>MATETTKMIYTPPPLDIKMEIEIGEQPQPPVKCSNFFANHWKGLVVFLVPLLCLPVMLLNEGAEFRCMYLLLVMAIFWVTEALPLYVTSMIPIVAFPIMGIMSSDQTCRLYFKDTLVMFMGGIMVALAVEYCNLHKRLALRVIQIVGCSPRRLHFGLIMVTMFLSMWISNAACTAMMCPIIQAVLEELQAQGVCKINHEPQYQIVGGNKKNNEDEPPYPTKITLCYYLGIAYASSLGGCGTIIGTATNLTFKGIYEARFKNSTEQMDFPTFMFYSVPSMLVYTLLTFVFLQWHFMGLWRPKSKEAQEVQRGREGADVAKKVIDQRYKDLGPMSIHEIQVMILFIFMVVMYFTRKPGIFLGWADLLNSKDIRNSMPTIFVVVMCFMLPANYAFLRYCTRRGGPVPTGPTPSLITWKFIQTKVPWGLVFLLGGGFALAEGSKQSGMAKLIGNALIGLKVLPNSVLLLVVILVAVFLTAFSSNVAIANIIIPVLAEMSLAIEIHPLYLILPAGLACSMAFHLPVSTPPNALVAGYANIRTKDMAIAGIGPTIITIITLFVFCQTWGLVVYPNLNSFPEWAQIYAAAALGNKTH[2x]

The I’m Not Dead Yet (INDY) protein in Drosophila melanogaster is a homodimeric plasma membrane transporter composed of 590 amino acids, belonging to the family of divalent anion–sodium symporters (DASS). INDY recognizes intermediates from the tricarboxylic acid cycle as substrates, with a preference for the dicarboxylate form of citrate at pH 6, and the anion exchanger inhibitor, DIDS (4,4′-diisothiocyano-2,2′-disulfonic acid stilbene), strongly inhibits its transport activity. Therefore, our biochemical characterization confirmed that INDY is a DIDS-sensitive H+/citrate symporter that predominantly recognizes citrate in its divalent form. Each protomer was divided into two domains: a central scaffold domain (TM 1–4 and 8–10), which plays an indispensable role in stable dimerization of the transporter, and a peripheral transport domain (HP1, HP2, TM 5–7, and TM 11–13) responsible for citrate binding and transport.

Apo-state structures of INDY were determined under two conditions: using nanodiscs at pH 6 and 8. The apo structures occurred in three conformations: (i) outward-open and (ii) inward-open conformations in which the substrate-binding site is exposed to the extracellular and intracellular sides, respectively, and (iii) an asymmetric conformation containing elements of both conformations. At pH 6, INDY exhibits two of these conformations, outward-open (43%) and asymmetric (57%). The ability of INDY to adopt multiple configurations in the apo state highlights the intrinsic dynamics of the transporter independent of substrate binding. Furthermore, the existence of an asymmetric conformation suggests that the two transport domains of INDY can slide independently across the membrane via an elevator-type mechanism. Furthermore, the two protomers move independently across the membrane.>[4x]DVDECALGANPCEHAGKCLNTLGSFECQCLQGYTGPRCEIDVNECISNPCQNDATCLDQIGEFQCICMPGYEGVYCEINTDECASSPCLHNGRCVDKINEFLCQCPKGFSGHLCQSGRLEVLFQ;>SSSIFQLRLQEFANERGMLANGRPCEPGCRTFFRICLKHYQATFSEGPCTFGNVSTPVLGTNSFVIRDKNSGSGRNPLQLPLNFTWPGTFSLNIQAWHTPGDDLRPETSPGNSLISQIIIQGS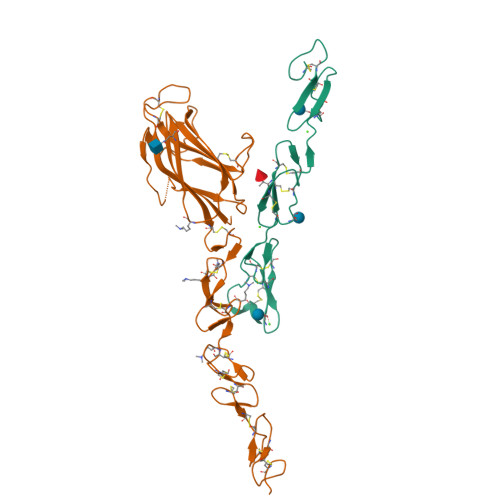LAVGKNWKSDEQNNTLTRLRYSYRVVCSDNYYGDSCSRLCKKRDDHFGHYECQPDGSPSCLPGWTGKYCDQPICLSGCHEQNGYCSKPDECNCRPGWQGPLCNECIPHKGCRHGTCTIPWQCACDEGWGGLFCDQAAA[4x]>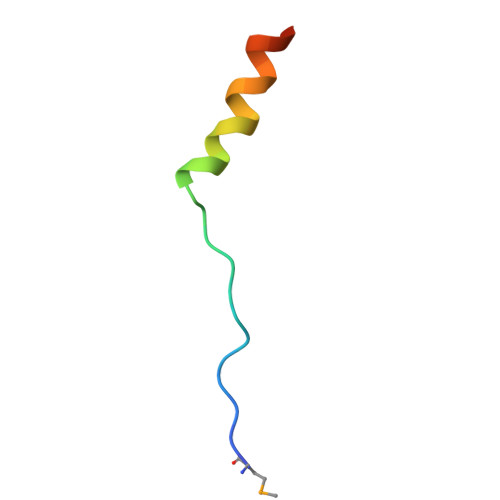 MLRRKPTRLELKLDDIEEFENIRKDLETR> VPDPRGIIINLDEGELCLNSAQCKSNCCQHDTILSLSRCALKARENSECSAFTLYGVYYKCPCERGLTCEGDKSLVGSITNTNFGICHNVGR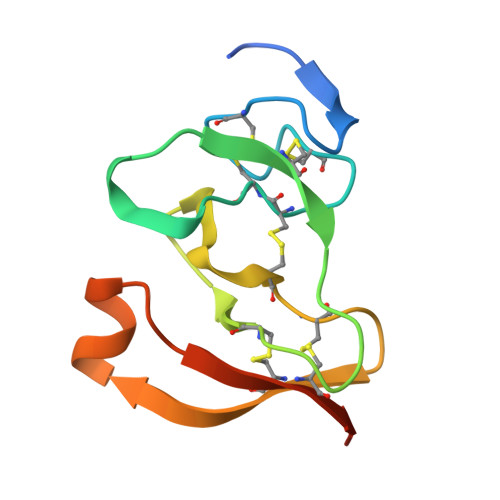SDS1H-benzimidazol-2-yl(1H-pyrrol-2-yl)methanone | C12 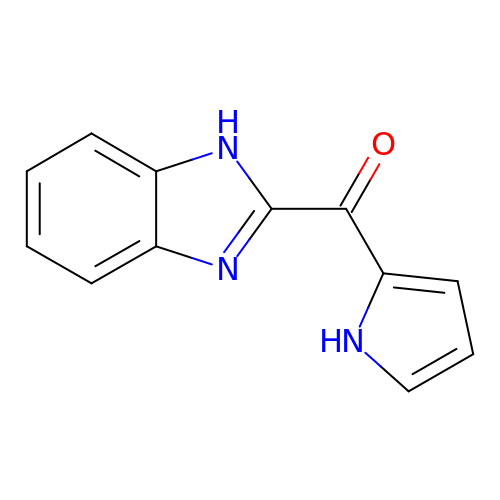H9 N3 O | WKGKIJSPPFRZEQ-UHFFFAOYSA-N> APGDPRECPGLLKGVYQSEHLFESDHQSGAWCKDPLQASDKIYYMPWTPYRTDTLTEYSSKDDFIAGRPTTTYKLPHRVDGTGFVVYDGALFFNKERTRNIVKFDLRTRIKSGEAIIANANYHDTSPYRWGGKSDIDLAVDENGLWVIYATEQNNGKIVISQLNPYTLRIEGTWDTAYDKRSASNAFMICGILYVVKSVYEDDDNEATGNKIDYIYNTDQSKDSLVDVPFPNSYQYIAAVDYNPRDNLLYVWNNYHVVKYSLDFGPAAAHHHHHHH;> APGDPREKSCPSVCRCDAGFIYCNDRFLTSIPTGIPEDATTLYLQNNQINNAGIPSDLKNLLKVERIYLYHNSLDEFPTNLPKYVKELHLQENNIRTITYDSLSKIPYLEELHLDDNSVSAVSIEEGAFRDSNYLRLLFLSRNHLSTIPWGLPRTIEEL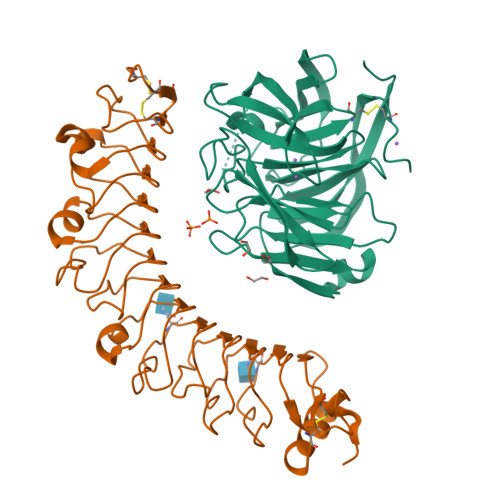RLDDNRISTISSPSLQGLTSLKRLVLDGNLLNNHGLGDKVFFNLVNLTELSLVRNSLTAAPVNLPGTNLRKLYLQDNHINRVPPNAFSYLRQLYRLDMSNNNLSNLPQGIFDDLDNITQLILRNNPWYCGCKMKWVRDWLQSLPVKVNVRGLMCQAPEKVRGMAIKDLNAELFDCKDSAAAHHHHHHH> SGNAFPGDTRILVQINGTPQRVTLKELYELFNEEHYESMVYVRKKPKVDIKVYSFNPEEGKVVLTDIEEVIKAPATDHLIRFELELGSSFETTVDHPVLVYENGKFVEKRAFEVREGNIIIIIDEST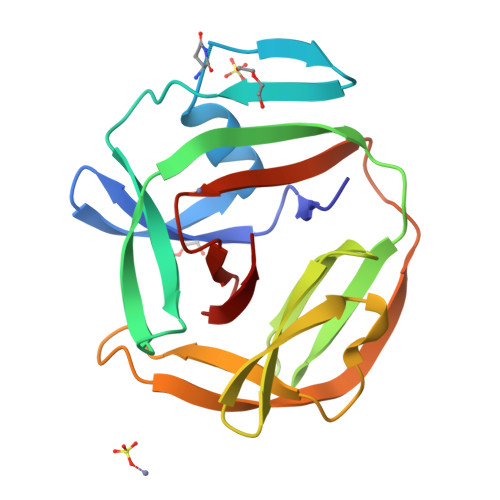LEPLKVAVKKIEFIEPPEDFVFSLNAKKYHTVIINENIVTHQ2-[3'-(hydroxymethyl)-1-methyl-5-({5-[(2S)-2-methyl-4-(oxetan-3-yl)piperazin-1-yl]pyridin-2-yl}amino)-6-oxo[1,6-dihydro[3,4'-bipyridine]]-2'-yl]-7,7-dimethyl-3,4,7,8-tetrahydro-2H-cyclopenta[4,5]pyrrolo[1,2-a]pyrazin-1(6H)-one | C37 H44 N8 O4 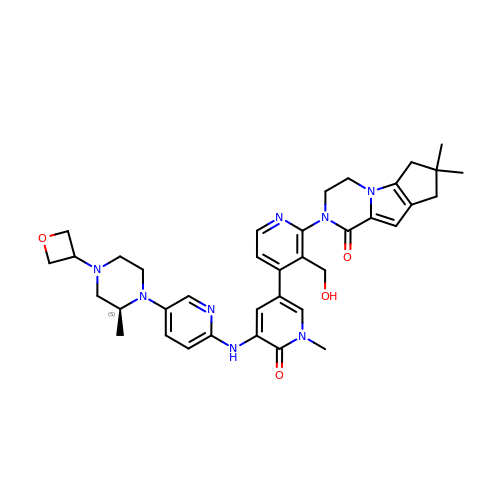| WNEODWDFDXWOLU-QHCPKHFHSA-N> MRGAPTYATALGSACLPFALDCDAILQASRRYSSTSAHGARSSAAASTSKLNYYRNLGVDTDATPQEVKTAYRQLALKYHPDVVEETHRAHAEMLFRRVSEAYEVLSDPVRRRAHDAELGIQTRRKQQPSATAPAGAPSAANAKAGTRAGSPAGGARPSSAFAERRKHTSSTASSTSSTTFQQQQQQQRRRYRKPFVRGDANRVFSDAFDGKTLDEILFDVQRRRRQEKAGRVAAERRHEKGGGAGHAASNGTTKSSSSPQPLMGESGPLDHDARLRHVMETAAELFAQRAQRQYGHGVLRHIRGVAGPLPDGPAPPPEVYMPFRPFVGMPVPPGVRTPPEPTLGKVLDSQEATVDSSSTPASRDAAWYEIPTQFHTHTYADGTPQSRSASLAKATKYIHGMPHNMGQLYSYHRP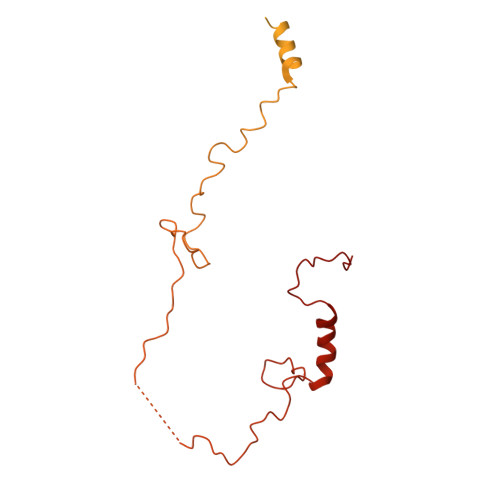Y>[4x]MGTTEDERR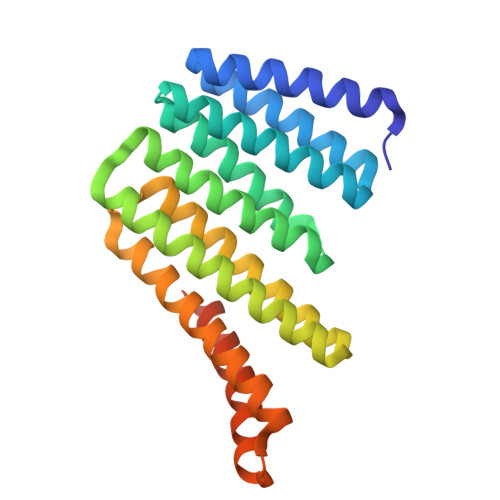ELEKVARKAIEAAREGNTDEVREQLQRALEIARESGTKTAVKLALDVALRVAQEAAKRGNKDAIDEAAEVVVRIAEESNNSDALEQALRVLEEIAKAVLKSEKTEDAKKAVKLVQEAYKAAQRAIEAAKRTGTPDVIKLAIKLAKLAARAALEVIKRPKSEEVNEALKKIVKAIQEAVESLREAEESGDPEKREKARERVREAVERAEEVQRDPSSGWLEHHHHHH>[8x]HMMSQQPPLRGSGDLGVLIERADGSVQILDGTAKTSLARVEGLGDLSH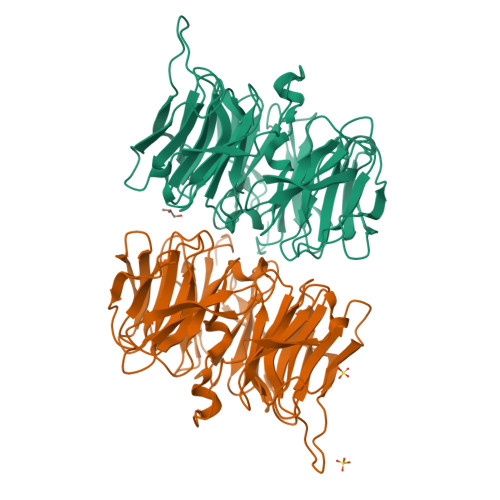ASLVFSRDQRYAYVFGRDGGLTKLDLLAQRIDKRLIQGGNSIGGAISQDGRLVAVSNYEPGGVKVFDSRTLELVAEIPATRLPGQDRNSRVVGLVDAPGQRFVFSLFDSGEIWIADFSQGDTPHLTRFRDIGKQPYDALISPDGRYYMAGLFGEDGMAQLDLWHPERGVRRVLGDYGRGQRKLPVYKMPHLEGWTIASDQAFVPAVGHHQVLVLDARDWKQTDAIDVAGQPVFVMTRPDDRQIWVNFAYPDNDKVQVIDSETHEVIETLRPGPGVLHMEFSGRGDQVWISVRDADQLQVWDPYRLKRIGSLPARSPSGIFFSHRAQHIGL>MSTADALDDENTFKILVATDIHLGFMEKDAVRGNDTFVTLDEILRLAQENEVDFILLGGDLFHENKPSRKTLHTCLELLRKYCMGDRPVQFEILSDQSVNFGFSKFPWVNYQDGNLNISIPVFSIHGNNDDPTGADALCALDILSCAGFVNHFGRSMSVEKIDISPVLLQKGSTKIALYGLGSIPDERLYRMFVNKKVTMLRPKEDENSWFNLFVIHQNRSKHGSTNFIPEQFLDDFIDLVIWGHEHECKIAPTKNEQQLFYISQPGSSVVTSLSPGEAVKKHVGLLRIKGRKMNMHKIPLHTVRQFFMEDIVLANHPDIFNPDNPKVTQAIQSFCLEKIEEMLENAERERLGNSHQPEKPLVRLRVDYSGGFEPFSVLRFSQKFVDRVANPKDIIHFFRHREQKEKTGEEINFGKLITKPSEGTTLRVEDLVKQYFQTAEKNVQLSLLTERGMGEAVQEFVDKEEKDAIEELVKYQLEKTQRFLKERHIDALEDKIDEEVRRFRETRQKNTNEEDDEVREAMTRARALRSQSEESASAFSADDLMSIDLAEQMANDSDDSISAATNKGRGRGRGRRGGRGQNSASRGGSQRGRADTGLETSTRSRNSKTAVSASRNMSIIDAFKSTRQQPSRNVTTKNYSEVIEVDESDVEEDIFPTTSKTDQRWSSTSSSKIMSQSQVSKGVDFESSEDDDDDPFMNTSSLRRNRRSGGSLEVLFQGPDYKDDDDKGTDYKDDDDK[2x];> MWKLLPAAGPAGGEPYRLLTGVEYVVGRKNCAILIENDQSISRNHAVLTANFSVTNLSQTDEIPVLTLKDNSKYGTFVNEEKMQNGFSRTLKSGDGITFGVFGSKFRIEYEPLVACSSCLDVSGKTALNQAILQLGGFTVNNWTEECTHLVMVSVKVTIKTICALICGRPIVKPEYFTEFLKAVESKKQPPQIESFYPPLDEPSIGSKNVDLSGRQERKQIFKGKTFIFLNAKQHKKLSSAVVFGGGEARLITEENEEEHNFFLAPGTCVVDTGITNSQTLIPDCQKKWIQSIMDMLQRQGLRPIPEAEIGLAVIFMTTKNYCDPQGHPSTGLKTTTPGPSLSQGVSVDEKLMPSAPVNTTTYVADTESEQADTWDLSERPKEIKVSKMEQKFRMLSQDAPTVKESCKTSSNNNSMVSNTLAKMRIPNYQLS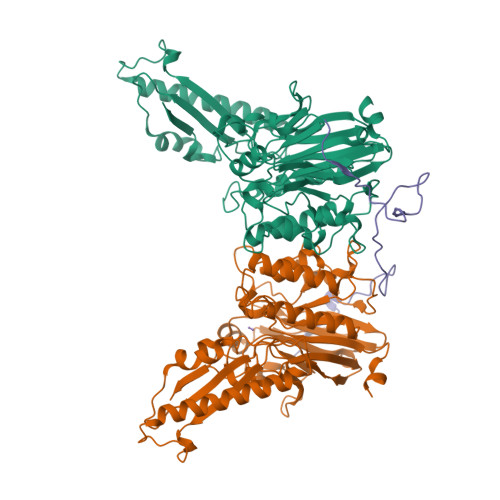PTKLPSINKSKDRASQQQQTNSIRNYFQPSTKKRERDEENQEMSSCKSARIETSCSLLEQTQPATPSLWKNKEQHLSENEPVDTNSDNNLFTDTDLKSIVKNSASKSHAAEKLRSNKKREMDDVAIEDEVLEQLFKDTKPELEIDVKVQKQEEDVNVRKRPRMDIETNDTFSDEAVPESSKISQENEIGKKRELKEDSLWSAKEISNNDKLQDDSEMLPKKLLLTEFRSLVIKNSTSRNPSGINDDYGQLKNFKKFKKVTYPGAGKLPHIIGGSDLIAHHARKNTELEEWLRQEMEVQNQHAKEESLADDLFRYNPYLKRRR> GAMDAAV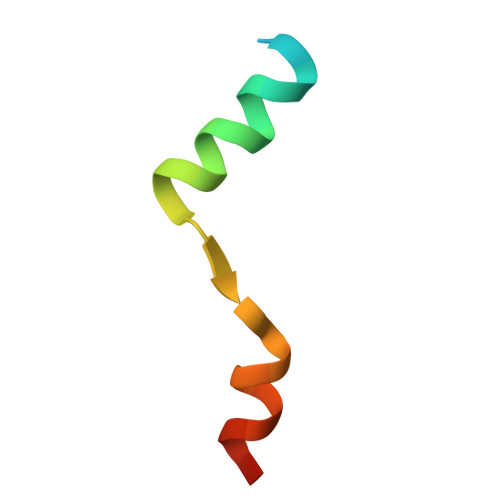APEERHLSKMQQNGYENPTYKFFEQMQN>HHHHHHGSEKWTSTAIITQPDVGQIAGYNNAMNVIYGQAAPKVSDLQETLIGRFSSAFSALAETLDNQEEPEKLTIEPSVKNQQLPLTVSYVGQTAEGAQMKLAQYIQQVDDKVNQELEKDLKDNIALGRKNLQDSLRTQEVVAQEQKDLRIRQIQEALQYANQAQVTKPQVQQTEDVTQDTLFLLGSEALESMIKHEATRPLVFSPNYYQTRQNLLDIEKLKFDDLDI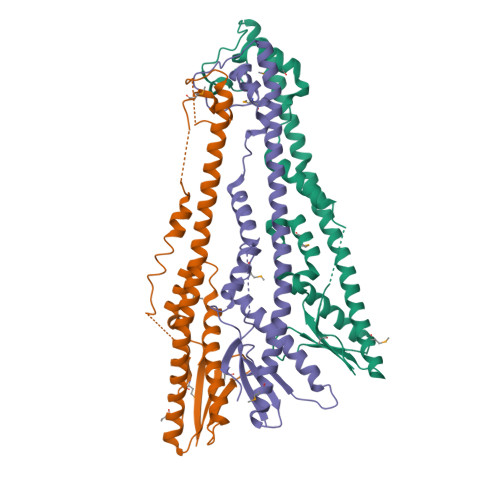HAYRYVMKPTL[3x]> PTV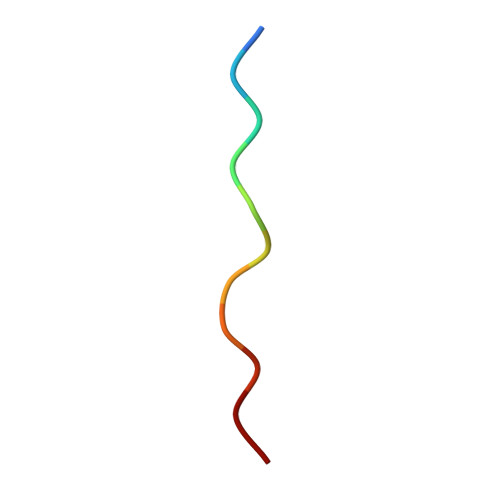APPAPVYR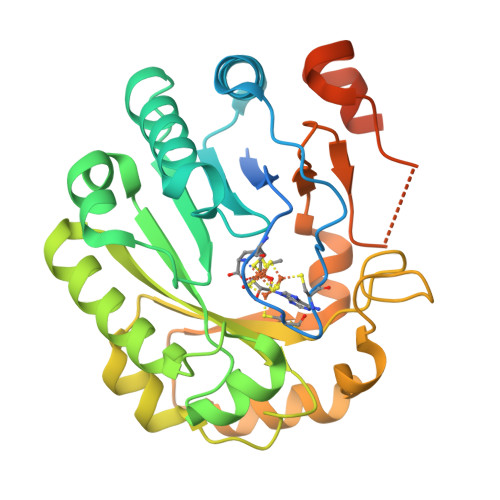>[2x]GKEQPQVRGELEETQETQEDGNSTQRTTPVSVNYHFTRQCNYKCGFCFHTAKTSFVLPLEEAKRGLLLLKQAGLEKINFSGGEPFLQDRGEYLGKLVRFCKEELALPSVSIVSNGSLIRERWFKDYGEYLDILAISCDSFDEQVNALIGRGQGKKNHVENLQKLRRWCRDYKVAFKINSVINRFNVDEDMNEHIKALSPVRWKVFQCLLIEGENSGEDALREAERFLISNEEFETFLERHKEVSCLVPESNQKMKDSYLILDEYMRFLNCTGGRKDPSKSILDVGVEEAIKFSGFDEKMFLKRGGKYVWSKADLKLDW>[14x]MSFPYFISPEQAMRERSELARKGIARAKSVVALAYAGGVLFVAENPSRSLQKISELYDRVGFAAAGKFNEFDNLRRGGIQFADTRGYAYDRRDVTGRQLANVYAQTLGTIFTEQAKPYEVELCVAEVAHYGETKRPELYRITYDGSIADEPHFVVMGGTTEPIANALKESYAENASLTDALRIAVAALRAGSADTSGGDQPTLGVASLEVAVLDANRPRRAFRRITGSALQALLVDQESPQSDGESSG;>ATIVALKYPGGVVMAGDRRSTQGNMISGRDVRKVYITDDYTATGIAGTAAVAVEFARLYAVELEHYEKLEGVPLTFAGKINRLAIMVRGNLAAAMQGLLALPLLAGYDIHASDPQSAGRIVSFDAAGGWNIEEEGYQAVGSGSLFAKSSMKKLYSQVTDGDSGLRVAVEALYDAADDDSATGGPDLVRGIFPTAVIIDADGAVDVPESRIAELARAIIESRSGADTFGSDGGEK[14x]

The Mycobacterium tuberculosis (Mtb) proteasome system selectively degrades damaged or misfolded proteins and is crucial for the pathogen’s survival within the host. Mtb 20S core particle features homoheptameric rings in a conserved α7-β7-β7-α7 configuration. These rings assemble to form three interconnected compartments: two antechambers formed by α7-β7 and a central degradation chamber. Stacked β-rings enclose the degradation chamber where active sites containing the catalytic triad of βT1, βD17, and βK33 proteolyze substrates.

Here we determine near-atomic resolution cryo-EM structures of Mtb 20S CP, revealing an auto-inhibited state, 20Sauto-inhibited, that interconverts with the canonical resting state, 20Sresting. These structures mainly differ in the conformation of a pair of β-subunit helices at α-β interface, which we have named switch helices I and II, following the convention established by Losick and coworkers. We subsequently fit our molecular models to the first and last intermediate reconstructed maps and achieved excellent refinement statistics. Frames 1 and 20 represent the most distinct states in the continuum. The initial frame closely resembles our modelled inactive consensus structure of 20SβT1A (RMSD 0.44 Å), featuring additional conformational changes in switch helix II. The S1 pocket and the conformation of the catalytic residues are unchanged. This represents an observation of an auto-inhibited conformation of the switch helices in Mtb 20S CP, which we will refer to as 20Sauto-inhibited. Additionally, we explored the C terminus of switch helix II, which shows unwinding in 20Sauto-inhibited. The preceding residues are disordered in the 20Sauto-inhibited state. Molecules that selectively bind to and stabilize the 20Sauto-inhibited of the proteasome established in this study, rather than the well-known canonical resting state (20Sresting) could be critical to future inhibitor development efforts that focus on allosteric rather than orthosteric sites of Mtb 20S CP.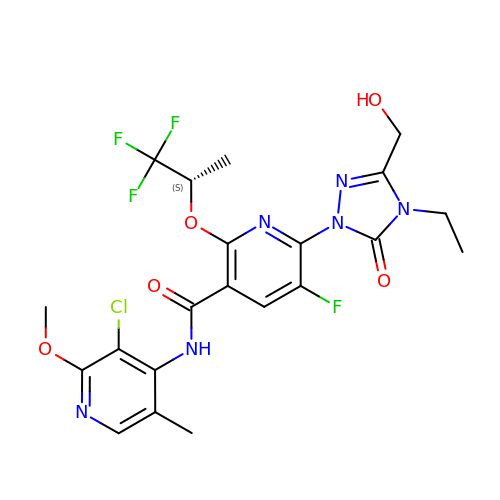(6M)-N-(3-chloro-2-methoxy-5-methylpyridin-4-yl)-6-[4-ethyl-3-(hydroxymethyl)-5-oxo-4,5-dihydro-1H-1,2,4-triazol-1-yl]-5-fluoro-2-{[(2S)-1,1,1-trifluoropropan-2-yl]oxy}pyridine-3-carboxamide | C21 H21 Cl F4 N6 O5 | FJYNLQXYLQBCRQ-JTQLQIEISA-N>MRAVFFDLDNTLIDTAGASRRGMLEVIKLLQSKYHYKEEAEIICDKVQVKLSKECFHPYNTCITDLRTSHWEEAIQETKGGAANRKLAEECYFLWKSTRLQHMTLAEDVKAMLTELRKEVRLLLLTNGDRQTQREKIEACACQSYFDAVVVGGEQREEKPAPSIFYYCCNLLGVQPGDCVMVGDTLETDIQGGLNAGLKATVWINKNGIVPLKSSPVPHYMVSSVLELPALLQSIDCLVPR[2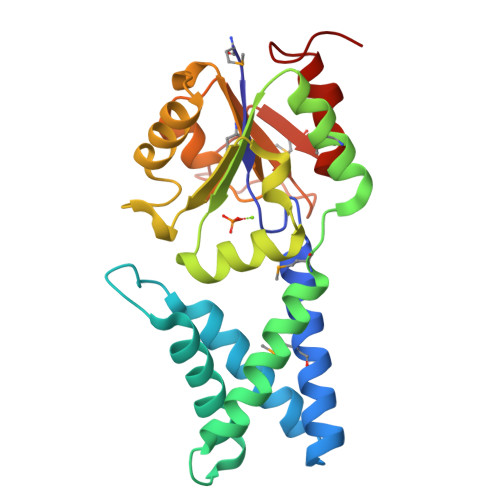x]> SRLQELAVIPILVIACDRSTVRRCLDKLLHYRPSAELFPIIVSQDCGHEETAQVIASYGSAVTHIRQPDLSNIAVQPDHRKFQGYYKIARHYRWALGQIFHNFNYPAAVVVEDDLEVAPDFFEYFQATYPLLKADPSLWCVSAWNDNGKEQMVDSSKPELLYRTDFFPGLGWLLLAELWAELEPKWPKAFWDDWMRRPEQRKG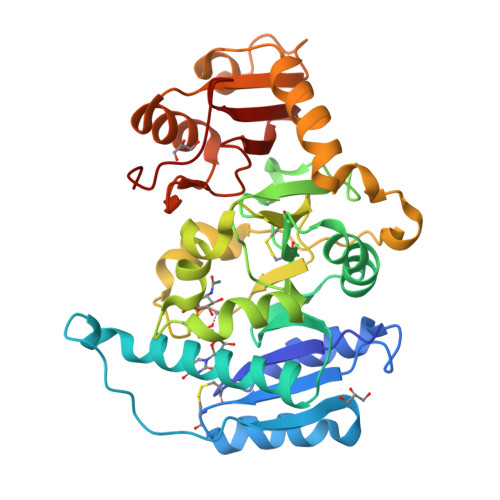RACVRPEISRTMTFGRKGVSHGQFFDQHLKFIKLNQQFVPFTQLDLSYLQQEAYDRDFLARVYGAPQLQVEKVRTNDRKELGEVRVQYTGRDSFKAFAKALGVMDDLKSGVPRAGYRGIVTFLFRGRRVHLAPPQTWDGYDPSWT N-(3-bromo-4-fluorophenyl)-N'-hydroxy-4-{[2-(sulfamoylamino)ethyl]sulfanyl}-1,2,5-oxadiazole-3-carboximidamide 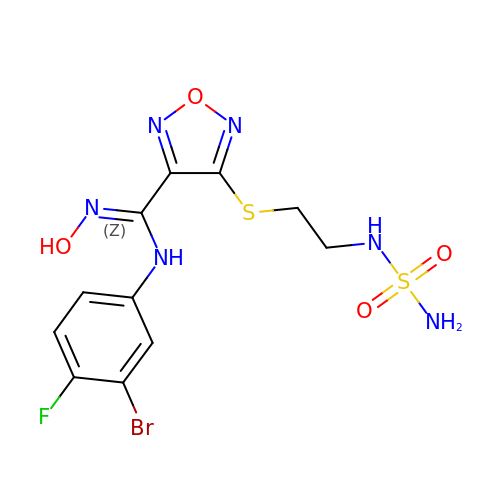| C11 H12 Br F N6 O4 S2 | WSIGGURFGMNQNZ-UHFFFAOYSA-N>[2x]MTSAEMTSPNNNSEHQAIAKMRTMIEGFDDISHGGLPIGRSTLVSGTSGTGKTLFSIQFLYNGIIEFDEPGVFVTFEETPQDIIKNARSFGWDLAKLVDEGKLFILDASPDPEGQ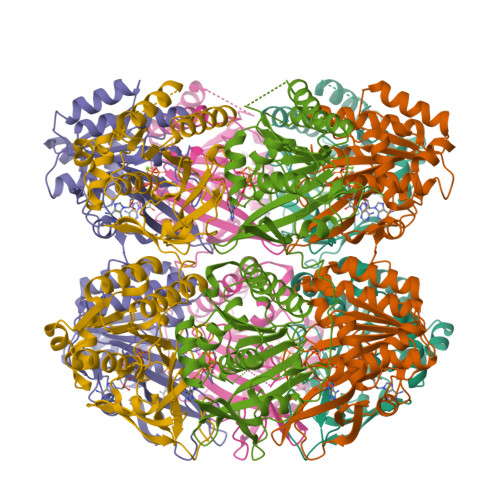EVVGGFDLSALIERINYAIQKYRARRVSIDSVTSVFQQYDASSVVRRELFRLVARLKQIGATTVMTTERIEEYGPIARYGVEEFVSDNVVILRNVLEGERRRRTLEILKLRGTSHMKGEYPFTITDHGINIFPLGAMRLTQRSSNVRVSSGVVRLDEMCGGGFFKDSIILATGATGTGKTLLVSRFVENACANKERAILFAYEESRAQLLRNAYSWGMDFEEMERQNLLKIVCAYPESAGLEDHLQIIKSEINDFKPARIAIDSLSALARGVSNNAFRQFVIGVTGYAKQEEITGLFTNTSDQFMGAHSITDSHIAAITDTIILLQYVEIRGEMSRAINVFKMRGSWHDKAIREFMISDKGPDIKDSFRNFERIISGSPTRITVDEKSELSRIVRGVQEKGPES> MSNKVKTKA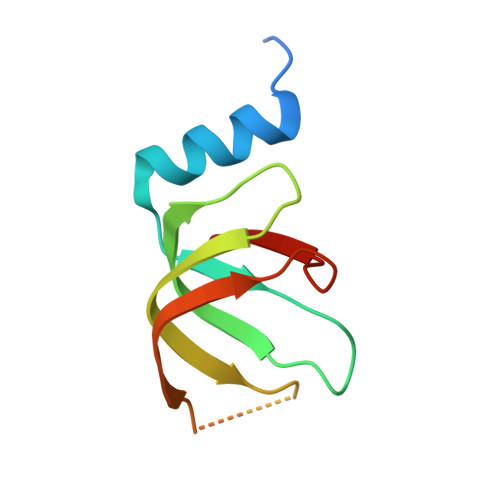MVPPINCIFNFLQQQTPVTIWLFEQIGIRIKGKIVGFDEFMNVVIDEAVEIPVNSADGKEDVEKGTPLGKILLKGDNITLITSAD> XSAVKAARYGKDNVRVYKVHKDEKTGVQTVYEMTVCVLLEGEIETSYTKADNSVIVATDSIKNTIYITAK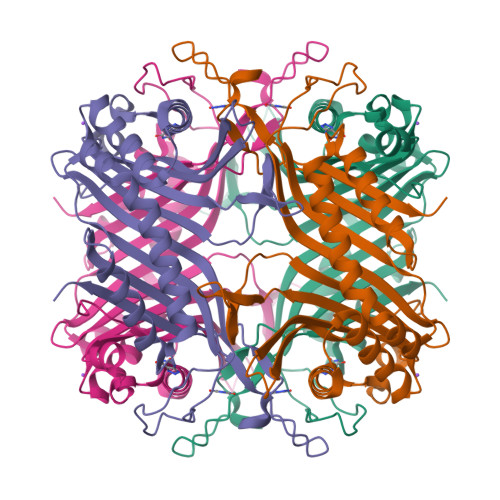QNPVTPPELFGSILGTHFIEKYNHIHAAHVNIVCHRWTRMDIDGKPHPHSFIRDSEEKRNVQVDVVEGKGIDIKSSLSGLTVLKSTNSQFWGFLRDEYTTLKETWDRILSTDVDATWQWKNFSGLQEVRSHVPKFDATWATAREVTLKTFAEDNSASVQATMYKMAEQILARQQLIETVEYSLPNKHYFEIDLSWHKGLQNTGKNAEVFAPQSDPNGLIKCTVGRSSLKSKL>GAMGRRPEEWGKLIYQWVSRSGQNNSVFTLYELTNGEDTEDEEFHGLDEATLLR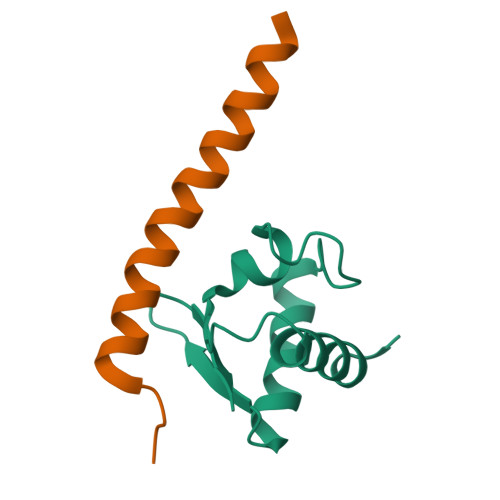ALQALQQEHKAEIITVSDGRGVKFF[4x];>GSRVTEQDKAILQLKQQRDKLRQYQKRIAQQLERERALA[4x]> MQVLHVCSEMFPLLKTGGLADVIGALPAAQIADGVDARVLLPAFPDIRRGVTDAQVVSRRDTFAGHITLLFGHYNGVGIYLIDAPHLYDRPGSPYHDTNLFAYTDNVLRFALLGWVGAEMASGLDPFWRPDVVHAHDWHAGLAPAYLAARGRPAKSVFTVHNLAYQGMFYAHHMNDIQLPWSFFNIHGLEFNGQISFLKAGLYYADHITAVSPTYAREITEPQFAYGMEGLLQQRHREGRLSGVLNGVDEKIWSPE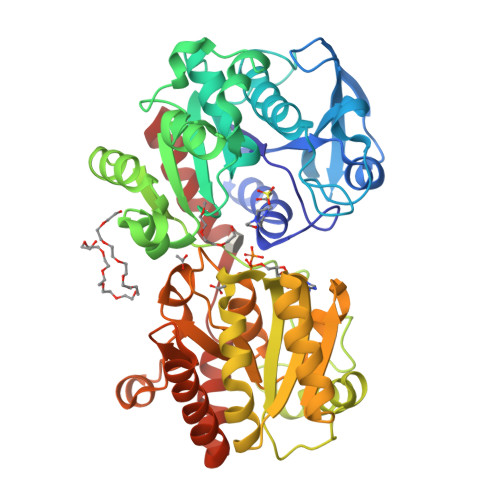TDLLLASRYTRDTLEDKAENKRQLQIAMGLKVDDKVPLFAVVSRLTSQKGLDLVLEALPGLLEQGGQLALLGAGDPVLQEGFLAAAAEYPGQVGVQIGYHEAFSHRIMGGADVILVPSRFEPCGLTQLYGLKYGTLPLVRRTGGLADTVSDCSLENLADGVASGFVFEDSNAWSLLRAIRRAFVLWSRPSLWRFVQRQAMAMDFSWQVAAKSYRELYYRLKLEHHHHHH>MMYRAPKTEKGKESLNKILDASVELIADKGFLSTSINDITSKAGVAYGLFYFYFKSKHDILDEIIRQFNRNMRYYLKTYTQNLDSRIDVEKVGMKKFLEWMNENKKYYKIFIETQVHRPDIYKWHFMKLAERYTTGLSEAMRRGEIINVDP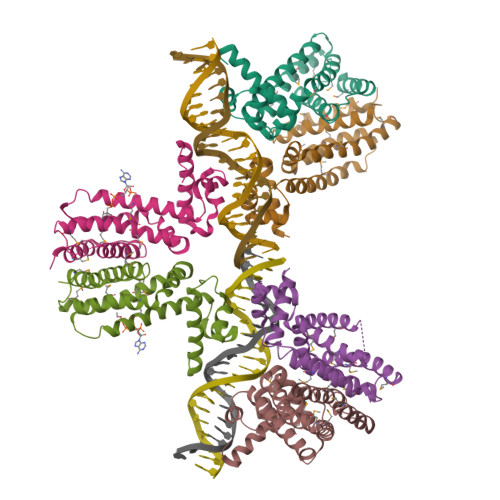ELLSYVLIGIAHMLGKRYVLWSNSGLTLKQQRDLDLIIENMLTPR[6x]> SQIEWAKA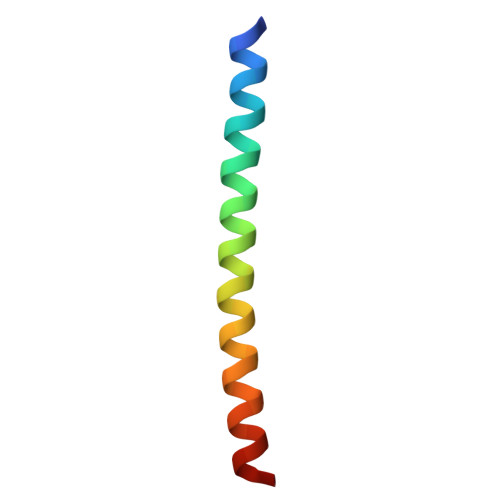RVEKLRKRNQALKSQTSELQRQIAELEASNAELKK>MAFELPKLPYAFDALEPHFDKETMEIHHDRHHNTYVTKLNAAVEGTDLESKSIEEIVANLDSVPANIQTAVRNNGGGHLNHSLFWELLSPNSEEKGTVVEKIKEQWGSLEEFKKEFADKAAARFGSGWAWLVVNNGQLEIVTTPNQDNPLTEGKTPILLFDVWEHAYYLKYQNKRPDYIGAFWNVVNWEKVDELYNATK[2x]

SODs detoxify superoxide, a reactive oxygen radical produced by aerobic metabolism and by the mammalian immune system in response to infection. We recently established that a Mn/Fe SOD from the bacterium Staphylococcus aureus exhibits equal activity with either manganese or iron. In addition to the camSOD (SodM), S. aureus also possesses a second, manganese-dependent SOD (SodA). All members of the Mn/Fe SOD family are related in sequence, exhibit identical protein folds, and coordinate their metal ion using identical ligands, making it unclear why some enzymes absolutely require manganese for catalysis (MnSOD), while others require iron (FeSOD), and still others show metal cofactor flexibility (camSOD).

Remarkably, the chemical differences between the sidechains of these residues are minor, with Gly (MnSOD) and Leu (camSOD) at position 159, and Leu (MnSOD) and Phe (camSOD) at position 160. The MnSOD double mutant (Gly159Leu-Leu160Phe) showed a substantial difference in metal utilization from that of the wild type or the single-mutant variants. The iron-dependent activity of the MnSOD double mutant was increased >20-fold relative to wild-type MnSOD, resulting in a highly cambialistic enzyme that displayed activity with manganese and with iron that differed only ~2-fold (CR = 0.486). It’s notable that, like in wild-type camSOD, this highly cambialistic variant exhibited diminished activity with manganese, illustrating that gaining cofactor flexibility requires a compromise with catalytic efficiency. The camSOD triple mutant (Ile19Phe-Leu159Gly-Phe160Leu) had increased activity with both metals relative to the double mutant (camSOD Leu159Gly-Phe160Leu). These studies demonstrate that positions 159 and 160 are important in regulating the reactivity of the metal cofactor. Strikingly, mutations at these positions produced profound effects on metal specificity, yet did so with essentially no changes to the protein backbone structure, at least within the resolution of the crystal structures. Altogether, the spectroscopic data indicate that the two wild-type S. aureus SODs and the two double mutants differ in their manganese redox properties. The auto-oxidation data and dithionite reduction data both suggest that the two wild-type SODs have different reduction potentials. These differences are inverted in the double mutants in both assays, which correlates with the inversion of manganese-dependent activity in these variants. The double mutation in MnSOD resulted in an altered electronic structure and re-tuning of the manganese reduction potential to more closely match that of camSOD and more catalytically active with iron, whereas the camSOD mutations altered reduction potential to make it more similar to MnSOD and more catalytically active with manganese.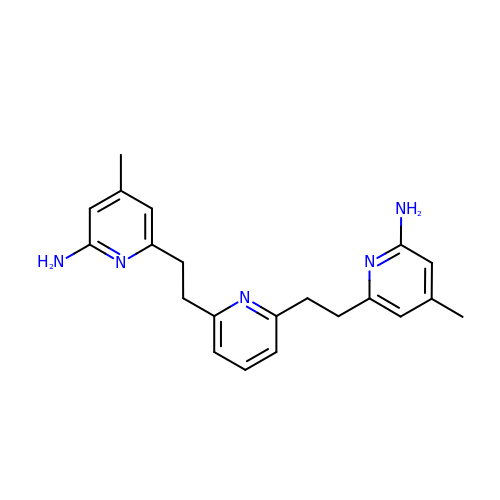6,6'-(pyridine-2,6-diyldiethane-2,1-diyl)bis(4-methylpyridin-2-amine) | C21 H25 N5 | NHAXZADCONDMKK-UHFFFAOYSA-N[(2R)-1-(L-ALANYL-L-ISOLEUCYL)PYRROLIDIN-2-YL]BORONIC 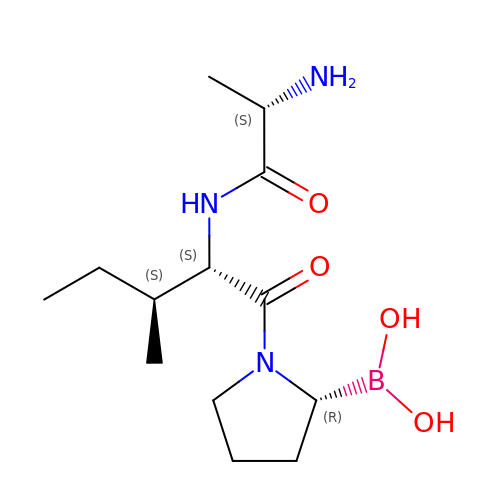ACID | C13 H26 B N3 O4 | ZJPVCZLCDXPKCH-NAKRPEOUSA-N>MLEISKVTPKAPPRYGWMNGQCIPWDQCSLHVSTQAAFFGASLFEGVRAYWNAEREQLYVFRLDEHLRRLEQSA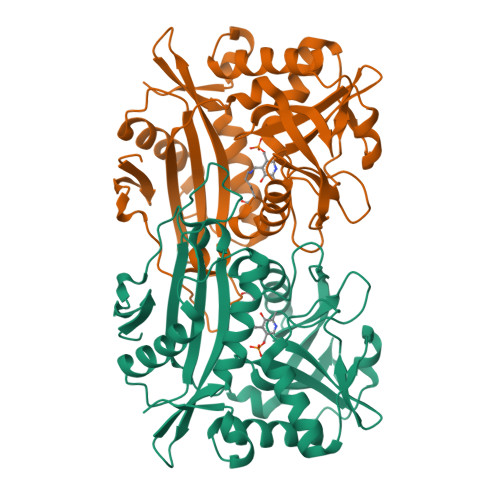KMLRMKLSMPIADIRQGVLELLRANEFRSDVHLYVASYFGINHDPDPLFPTDDTGVYVTGTAVSRLPLVHTGISACMSSWRRISDDSVPPRIKIGANYQNSRLAQTEARVNGYHTSVLLNSRGKVSETPGACLLMVRDGRVISPPVTADILESVTRKTLMSLSEAELDSPVIERDMDRTELYIAEEVFLCGTIAEILPVTTIDRIQVGDGEVGPVTRRLQELYFGVTSGQLEAYKSWLLPVYE[6x]> GSYPPPVFDFGMPRNITTRTGHTAAINCRVDNLGD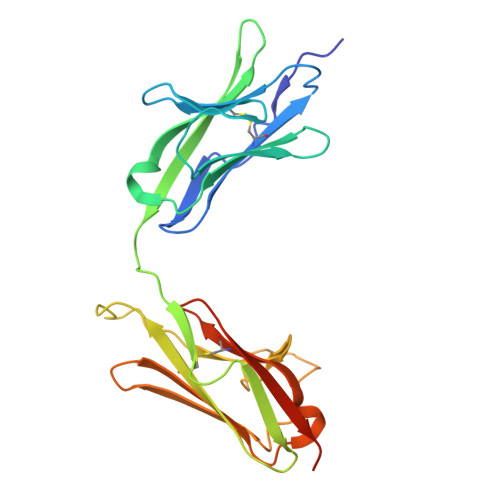KSVSWIRKRDLHILTAGILTYTSDERFKVVRTADSKDWTLHVKYAQPRDSGIYECQVNTEPKISMAFRLNVIVTPPDAKAIIAGPTDLYVKVGSSVTLTCHVKQPATSAQDIGPIYWYRGPYILTPFVAHPNDAAIDLQRISMESTLAEKLQSRLRIANAQLLDTGNYTCMPTTAEAASVVVNVINDEHHHHHHHH>[2x]MKVEEILEKALELVIPDEEEVRKGREAEEELRRRLDELGVEYVFVGSYARNTWLKGSLEIDVFLLFPEEFSKEELRERGLEIGKAVLDSYEIRYAEHPYVHGVVKGVEVDVVPCYKLKEPKNIKSAVDRTPFHHKWLEGRIKGKENEVRLLKGFLKANGIYGAEYKVRGFSGYLCELLIVFYGSFLETVKNAR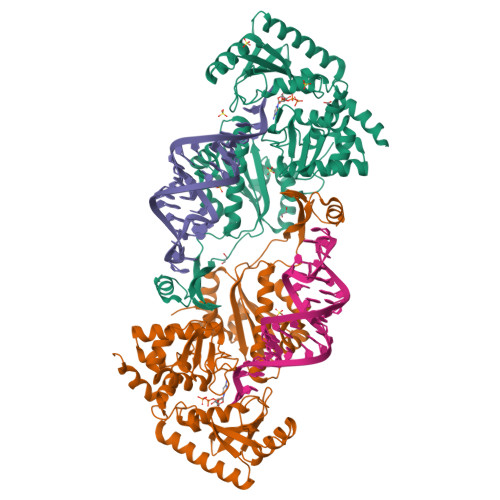RWTRRTVIDVAKGEVRKGEEFFVVDPVDEKRNVAANLSLDNLARFVHLCREFMEAPSLGFFKPKHPLEIEPERLRKIVEERGTAVFAVKFRKPDIVDDNLYPQLERASRKIFEFLERENFMPLRSAFKASEEFCYLLFECQIKEISRVFRRMGPQFEDERNVKKFLSRNRAFRPFIENGRWWAFEMRKFTTPEEGVRSYASTHWHTLGKNVGESIREYFEIISGEKLFKEPVTAELCEMMGVKDVCCM> EFMAIERTLSIVKPDAVSKNHIGEIFARFEKAGLKIVATKMKHLSQADAEGFYAEHKERGFFGDLVAFMTSGPVVVSVLEG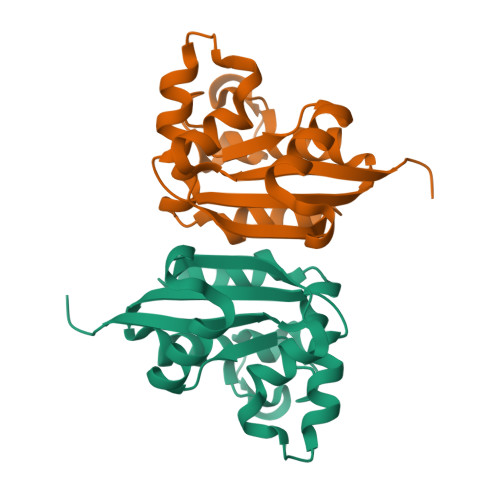ENAVLAHREILGATNPKEAAPGTIRADFAVSIDENAAHGSDSVASAEREIAYFFADNEICP Oxaziclomefone | C20 H19 Cl2 N O2 | 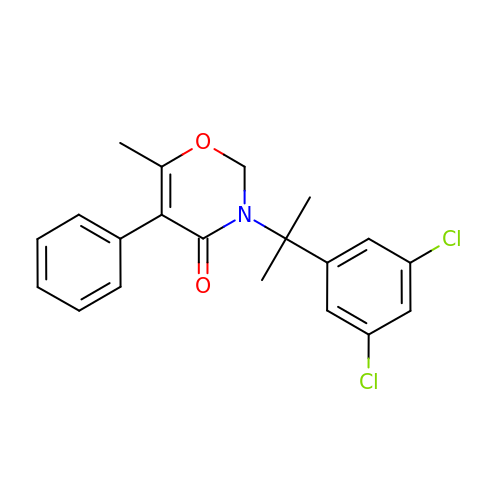FCOHEOSCARXMMS-UHFFFAOYSA-N4-[(3S,3aR,6S,6aR)-6-(3-methoxy-4-oxidanyl-phenyl)-1,3,3a,4,6,6a-hexahydrofuro[3,4-c]furan-3-yl]-2-methoxy-phenol 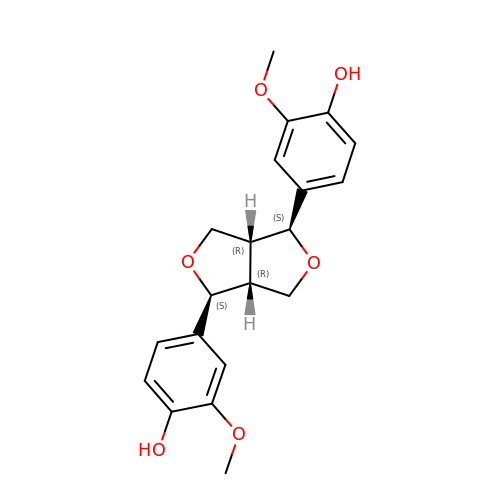| C20 H22 O6 | HGXBRUKMWQGOIE-AFHBHXEDSA-N>MTTLTARPEAITFDPQQSALIVVDMQNAYATPGGYLDLAGFDVSTTRPVIANIQTAVTAARAAGMLIIWFQNGWDEQYV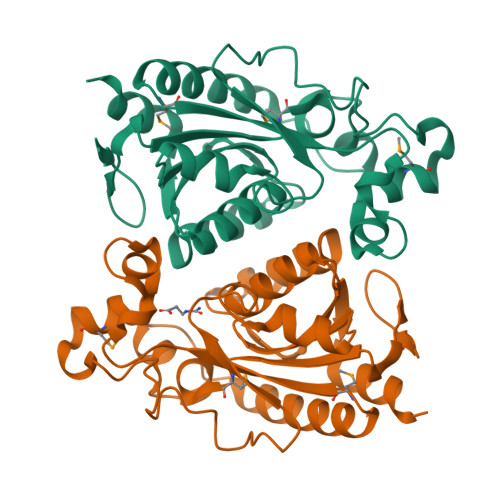EAGGPGSPNFHKSNALKTMRKQPQLQGKLLAKGSWDYQLVDELVPQPGDIVLPKPRYSGFFNTPLDSILRSRGIRHLVFTGIATNVCVESTLRDGFFLEYFGVVLEDATHQAGPKFAQKAALFNIETFFGWVSDVETFCDALSPTSFAHIA[16x]> FCPPAKVNILAQSRPLSEWPINLVSKGVQEYVYGLTAAEREANGDFGTSRKSLDRWFARTGVPTHGYTTVQGLNLILRHTFNRYDGVIKKVETRNEKRRSKATRINVSREADGLPPIEAEPEETAFGPDGKLKERPGINPSIYCYQQVSPVPYNPAKHPALPFSGVDPGAPLPLGTPNRLSIPKGQPGYVPEWQRPHLSTKNKRIRKWYARANWRRKPGRKSVLDEAKLKEAALKEAIPIIVTIGKDWIVMDARGLLRAVYWRGI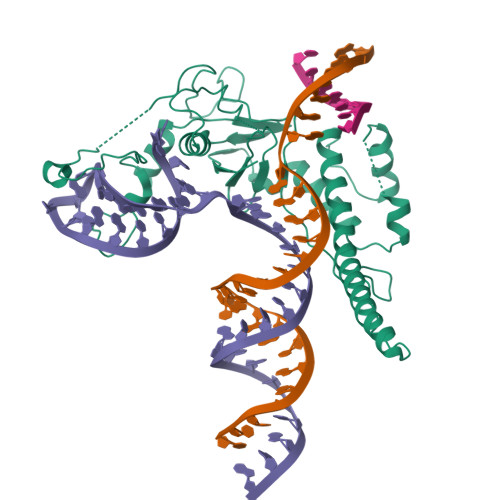AKPGLSLKELLGFFSGDPVLDPKRGIATFTFKLGA>[2x]NVKEKS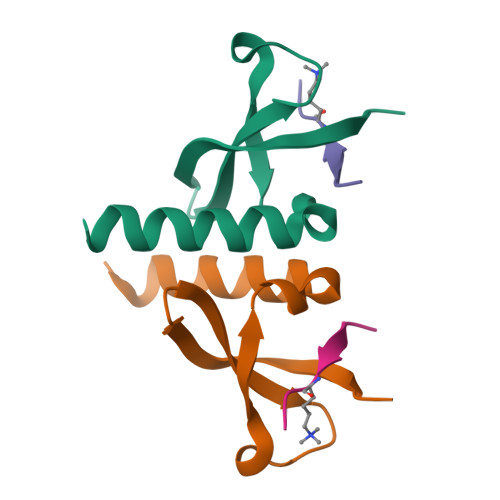SEYIVEKFLGKRYLRGRPQYLTKWEGYPIEQCTWEPLENLGKCMTLIADYEAELFQQSREKKNDQ;>[2x]KQTARKSTGGK> CQPIFLNVLEAIEPGVVCAGHDNNQPDSFAALLSSLNELGERQLVHVVKWAKALPGFRNLHVDDQMAVIQYSWMGLMVFAMGWRSFTNVNSRMLYFAPDLVFNEYRMHKSRMYSQCVRMRHLSQEFGWLQITPQEFLCMKALLLFSIIPVDGLKNQKFFDELRMNYIKELDRIIACKRKNPTSCSRRFYQLTKLLDSVQPIARE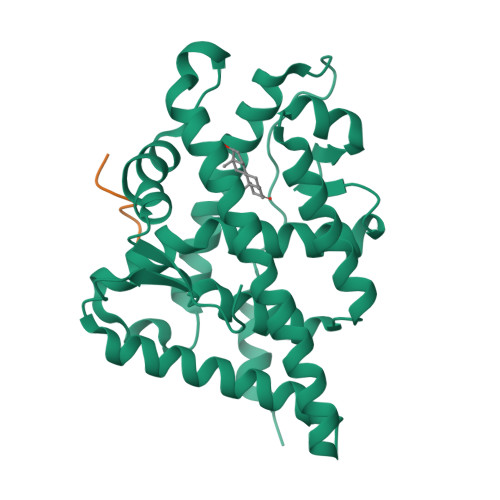LHQFTFDLLIKSHMVSVDFPEMMAEIISVQVPKILSGKVKPIYFHTQ;> KHKILHRLLQDSS>[3x]MVRTTKTSMAAASTVAPEVAMDEGSPSTSQAQVELPRNLEVFNEACGHVFGSSFNREDNSVISDAAAFLFKMHTHSLDGQEAKVLRASEKKRERENAKKSRKAPEAGMRVGRSLILTSRWTEYCATCVPALGSKMKVIKASGDAAMIQMMKDHNSLLRVCVRIEVWKARYVSLVALDERIQTLEDAQWFPYLSGDSYRACPGLVGGYFAKKAAAGERGKNYKKLNQTAIIPPPRFLIIGHR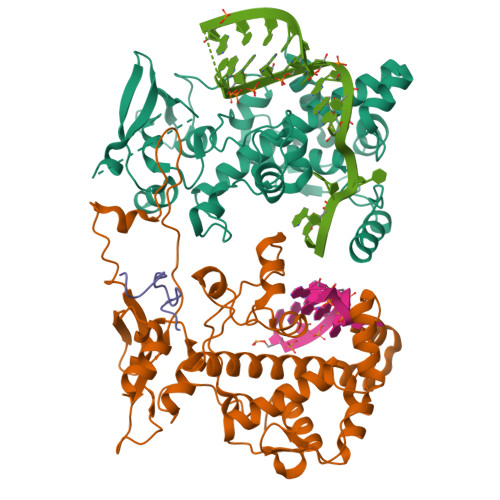LQIGDQVTLRELLASIAWGLCDGVLAECWSPSQGDGSIGVVVGLPLQATGSCFLVVASHGLSAIADSRIEGTGNTNLLEECIAIQKQDGVIKCKRSGKSLYHCLKETAGAVGR(3~{S})-1',1'-bis(chloranyl)-5-methyl-spiro[1~{H}-indole-3,2'-cyclopropane]-2-one | C11 H9 Cl2 N O | 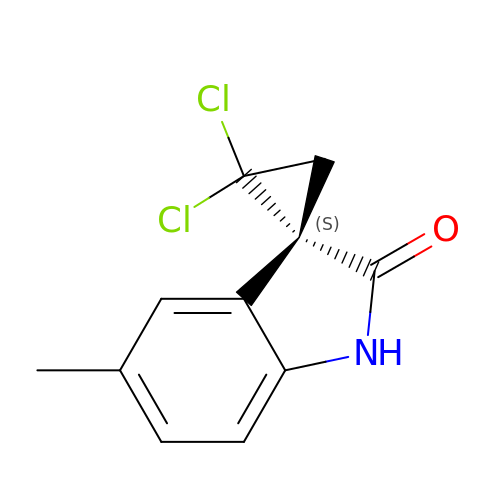ZLVLBGNQLFDEAB-JTQLQIEISA-N>GASGSGSGMLEVCIIGFGFSAIPLVRELARTQTEFQIISAESGSVWDRLSESGRLDFSLVSSFQTSFYSFDLVRDYEKDYYPTAKQFYEMHERWRSVYEEKIIRDFVTKIENFKDYSLISTRSGKTYEAKHVVLATGFDRLMNTFLSNFDNHVSNKTFVFDTMGDSANLLIAKLIPNNNKIILRTNGFTALDQEVQVLGKPFTLDQLESPNFRYVSSELYDRLMMSPVYPRTVNPAVSYNQFPLIRRDFSWVDSKSSPPNGLIAIKYWPIDQYYYHFNDDLENYISKGYLLNDIAMWLHTGKVILVPSDTPINFDKKTITYAGIERSFHQYVKGDAEQPRLPTILINGETPFEYLYRDTFMGVIPQRLNNIYFLGYTRPFTGGLANITEMQSLFIHKLITQPQFHQKIHQNLSKRITAYNQHYYGAAKPRKHDHTVPFGFYTEDIARLIGIHYQPNECRSVRDLLFYYAFPNNAFKYRLKGEYAVDGVDELIQKVNDKHDHYAQVFVQALSIRNMNSDEAAEWDHSARRFSFNDMRHKEGYRAFLDTYLKAYRQVENISVDDTVVDEEWNFMVKEACQVRDKVAPNIEEKTHYSKDEDVNKGIRLILSILDSDISSLPDSNGSRGSGNLKEGDRLCKFEAQSIEFIRRLLQPKNYELLFIRES[4x]

The flavin-dependent halogenase (FDH) AetF successively brominates tryptophan at C5 and C7 to generate 5,7-dibromotryptophan. In contrast to the well studied two-component tryptophan halogenases, AetF is a single-component flavoprotein monooxygenase. A large domain tightly binds the cofactor flavin adenine dinucleotide (FAD), while the small domain responsible for binding the nicotinamide adenine dinucleotide (NADP) is unoccupied. About half of the protein forms additional structural elements containing the tryptophan binding site.

The indole binding site is completed by the side chains of Glu200 and Thr373. The NH group of indole forms a hydrogen bond to the carbonyl of Met216. The amino group of Trp forms hydrogen bonds to the side-chain O atom of Gln500 and the carbonyl groups of both Leu199 and Leu215. The Trp carboxylate forms a salt bridge with Lys587 and hydrogen bonds to the side chains of both Gln500 and Ser523. Trp binds such that C5 is positioned correctly for halogenation. Rotational pseudo­symmetry and pseudomerohedral twinning complicated the phasing of one structure. All data sets for AetF soaked with Trp scaled well in point group 422 and showed a larger unit cell with a roughly doubled volume. Explicitly searching in P212121 gave a unique solution for four molecules per asymmetric unit with TFZ values of 19.5, 39.3, 41.1 and 101.6. The refined twin fraction for twin operator −h, −l, −k is 45%.>[8x]AEQVALSRTHVCGILREELFQGDAFHQSDTHIFIIMGASGDLAKKKIYPTIWWLFRDGLLPENTFIVGYARSRLTVADIRKQSEPFFKATPEEKLKLEDFFARNSYVAGQYDDAASYQRLNSHMNALHLGSQANRLFYLALPPTVYEAVTKNIHESCMSQIGWNRIIVEKPFGRDLQSSDRLSNHISSLFREDQIYRIDHYLGKEMVQNLMVLRFANRIFGPIWNRDNIACVILTFKEPFGTEGRGGYFDEFGIIRDVMQNHLLQMLCLVAMEKPAS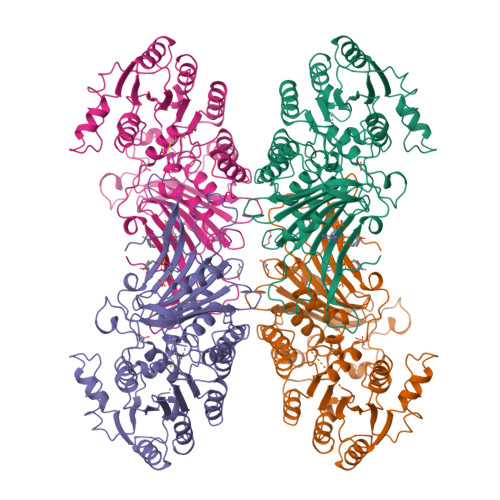TNSDDVRDEKVKVLKCISEVQANNVVLGQYVGNPDGEGEATKGYLDDPTVPRGSTTATFAAVVLYVENERWDGVPFILRCGKALNERKAEVRLQFHDVAGDIFHQQCKRNELVIRVQPNEAVYTKMMTKKPGMFFNPEESELDLTYGNRYKNVKLPDAYERLILDVFCGSQMHFVRSDELLEAWRIFTPLLHQIELEKPKPIPYIYGSRGPTEADELMKRVGFQYEGTYKWVNPHKL>[2x]SEGMEIDRGYISPQFVTNQERLLVE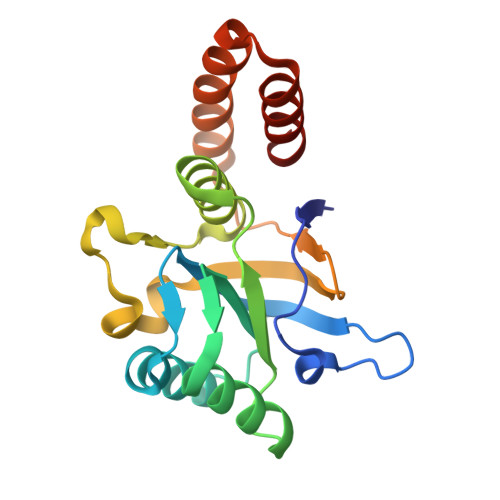YDNCRVLVTDQKIDAIRDIIPILEQVTRLNAPLLIIAEDVSGEALATLVVNKLRGVLNVCAIKAPGFGERRKSLLQDIAIVTGAEFIAKDLGMKVEQAVVEQLGVARKVTVANNTTTLIADAASKDEIEMRIAQLKKELAETDSVYDTEKLSERIAKLSGG>DTTTAHSDYEIILEGGSSSWGQVKGRAKVNVPAAIPLLPTDCNIRIDAKPLDAQKGVVRFTTKIESVVDSVKNTLNVEVDIANETKDRRIAVGEGSLSVGDFSHSFSFEGSVVNMYYYRSDAVRRNIPNPIYMQGRQFHDILMKVPLDNNDLVDTWEGFQQSISGGGANFGDWIREFWFIGPAFAAINEGGQRISPIVVNSSNVEGGEKGPVGVTRWKFSHAGSGVVDSISRWTELFPVEQLNKPASIEGGFRSDSQGIEVKVDGNLPGVSRDAGGGLRRILNHPLIPLVHHGMVGKFNDFTVDTQLKIVLPKGYKIRYAAPQFRSQNLEEYRWSGGAYARWVEHVCKGGTGQ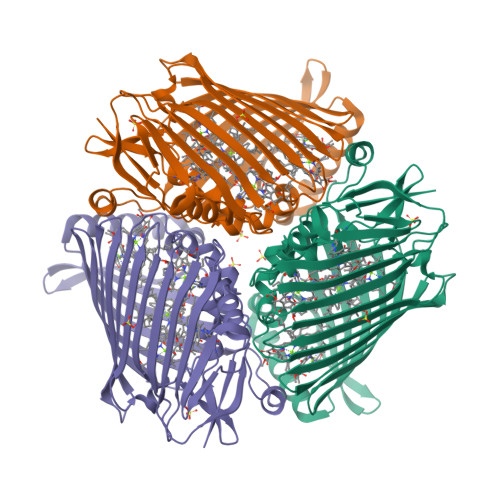FEVLYAQ[2x]>[2x]CPRFLKVKNWETDVVLTDTLHLKSTLETGCTEHICMGSIMLPSQHTRKPEDVA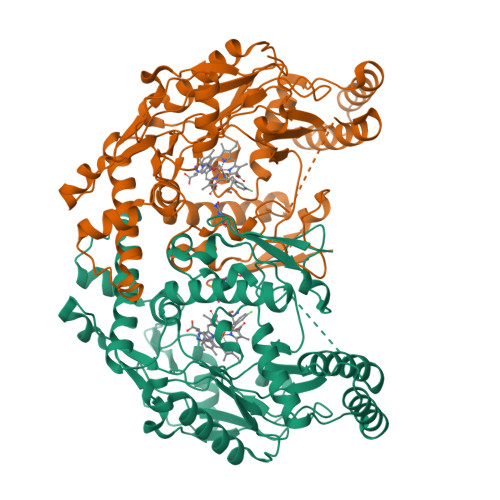TKDQLFPLAKEFLDQYYSSIKRFGSKAHMDRLEEVNKEIESTSTYQLKDTELIYGAKHAWRNASRCVGRIQWSKLQVFDARDCTTAHGMFNYICNHVKYATNKGNLRSAITIFPQRTDGKHDFRVWNSQLIRYAGYKQPDGSTLGDPANVQFTEICIQQGWKAPRGRFDVLPLLLQANGNDPELFQIPPELVLEVPIRHPKFDWFKDLGLKWYGLPAVSNMLLEIGGLEFSACPFSGWYMGTEIGVRDYCDNSRYNILEEVAKKMDLDMRKTSSLWKDQALVEINIAVLYSFQSDKVTIVDHHSATESFIKHMENEYRCRGGCPADWVWIVPPMSGSITPVFHQEMLNYRLTPSFEYQPDPWNTHVWKG> RHFDTY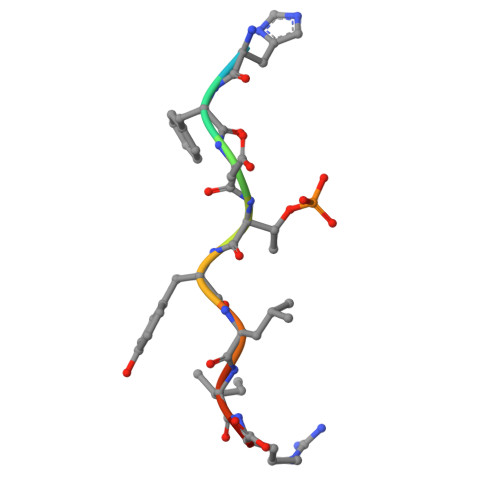LIRR> MRIPRIYHPEPLTSHSHIALCEDAANHIGRVLRMGPGQALQLFDGSNQVFDAEITSASKKSV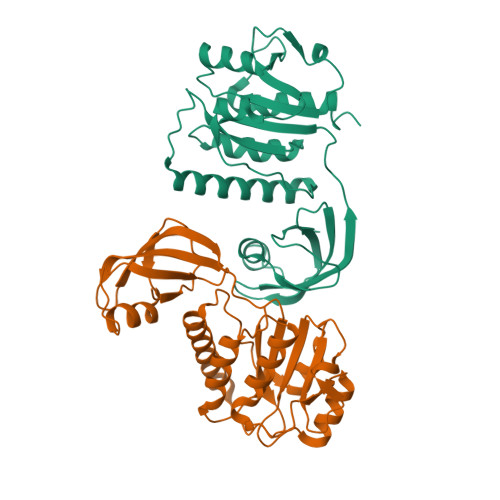EVKVLEGQIDDRESPLHIHLGQVMSRGEKMEFTIQKSIELGVSLITPLFSERCGVKLDSERLNKKLQQWQKIAIAACEQCGRNRVPEIRPAMDLEAWCAEQDEGLKLNLHPRASNSINTLPLPVERVRLLIGPEGGLSADEIAMTARYQFTDILLGPRVLRTETTALTAITALQVRFGDLGLEHHHHHH>[2x]GSMAQLGKLLKEQKYDRQLRLWGDHGQEALESAHVCLINATATGTEILKNLVLPGIGSFTIIDGNQVSGEDAGNNFFLQRSSIGKNRAEAAMEFLQELNSDVSGSFVEESPENLLDNDPSFFCRFTVVVATQLPESTSLRLADVLWNSQIPLLICRTYGLVGYMRIIIKEHPVIESHPDNALEDLRLDKPFPELREHFQSYDLDHMEKKDHSHTPWIVIIAKYLAQWYSETNGRIPKTYKEKEDFRDLIRQGILKPEDEENFEEAIKNVNTALNTTQIPSSIEDIFNDDRCINITKQTPSFWILARALKEFVAKEGQGNLPVRGTIPDMIADSGKYIKLQNVYREKAKKDAAAVGNHVAKLLQSIGQAPESISEKELKL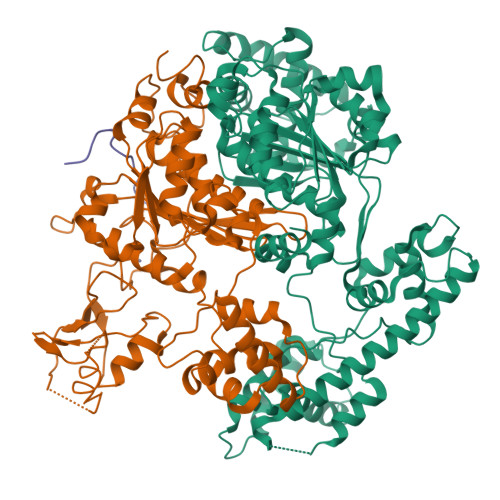LCSNSAFLRVVRCRSLAEEYGLDTINKDEIISSMDNPDNEIVLYLMLRAVDRFHKQQGRYPGVSNYQVEEDIGKLKSCLTGFLQEYGLSVMVKDDYVHEFCRYGAAEPHTIAAFLGGAAAQEVIKIITKQFVIFNNTYIYSGMSQTSATFQL;>MKLDWEGRWNHVKKFLERSGPFTHPDFEPSTESLQFLLDTCKVLVIGAGGLGCELLKNLALSGFRQIHVIDMDTIDVSNLNRQFLFRPKDIGRPKAEVAAEFLNDRVPNCNVVPHFNKIQDFNDTFYRQFHIIVCGLDSIIARRWINGMLISLLNYEDGVLDPSSIVPLIDGGTEGFKGNARVILPGMTACIECTLELYPPQVNFPMCTIASMPRLPEHCIEYVRMLQWPKEQPFGEGVPLDGDDPEHIQWIFQKSLERASQYNIRGVTYRLTQGVVKRIIPAVASTNAVIAAVCATEVFKIATSAYIPLNNYLVFNDVDGLYTYTFEAERKENCPACSQLPQNIQFSPSAKLQEVLDYLTNSASLQMKSPAITATLEGKNRTLYLQSVTSIEERTRPNLSKTLKELGLVDGQELAVADVTTPQTVLFKLHFTS[2x];>MIKLFSLKQQKKEEESAGGTKGSSKK[2x]> KRAH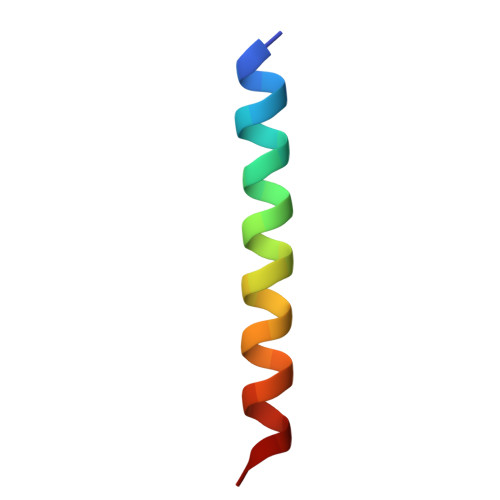HNALERKRRDHIKDSFHKLRDSVP> MAATTESVKADAAEA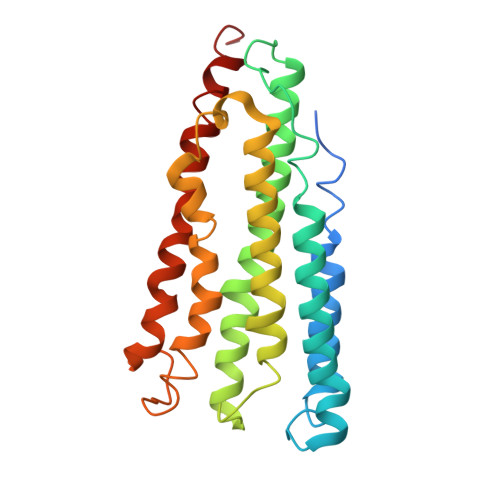PLLNKKNIIAGASLYLVFYAWVRWYEGVYGWSAGLDSFAPEFETYWMNFLYIEMVLEVLVASVLWGYIWKSRDRKVMSITPREELRRHFTHWTWLMMYGIAIYFGASYFTEQDGTWHQTIVRDTDFTPSHIIEFYLSYPIYIITGGASFLYAKTRLPTYQQGLSLQYLVVVVGPFMILPNVGLNEWGHTFWFMEELFVAPLHYGFVFFGWSALGVLGVINIELGALSKLLKKDLA>MRTEPLCGASPLLVPGDPYSVVVLLQGYAEPEGVGDAVRADGSVTLVLPQTRGPASSHRESPRGSGGA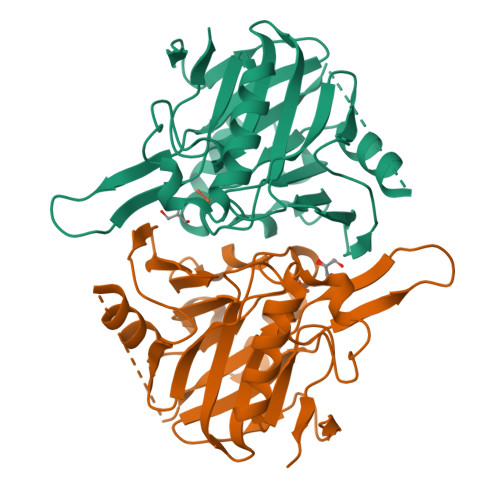EAALEEAARGPILVDTGGPWAREALLGALAGQGVAPGDVTLVVGTHGHSDHIGNLGLFPGAALLVSHDFCLPGGRYLPHGLGEGQPLRLGPGLEVWATPGHGGQRDVSVVVAGTALGTVVVAGDVFERDGDEDSWQALSEDPAAQERSRKRVLVVADVVVPGHGPPFRVLREASQPETEGGGNSQQEPVVGDEEPALH[4x]>MEKTTTQELLAQAEKICAQRNVRLTPQRLEVLRLMSLQDGAISAYDLLDLLREAEPQAKP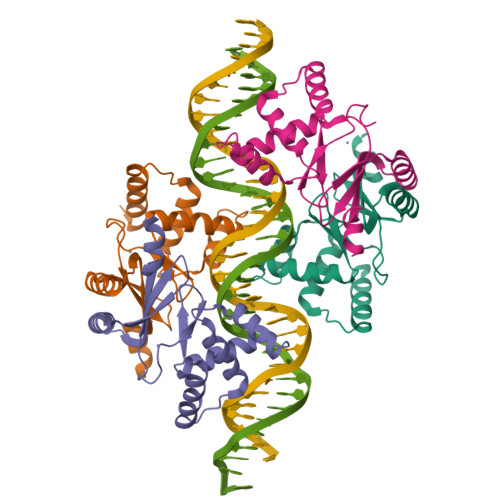PTVYRALDFLLEQGFVHKVESTNSYVLCHLFDQPTHTSAMFICDRCGAVKEECAEGVEDIMHTLAAKMGFALRHNVIEAHGLCAACVEVEACRHPEQCQHDHSVQVKKKPR[4x]>MSIITDVYAREILDSRGNPTIEVEVYTESGAFGRGMVPSGASTGEYEAVELRDGDKARYGGKGVTKAVDNVNNIIAEAIIGYDVRDQMAIDKAMIALDGTPNKGKLGANAILGVSIAVARAAADYLEVPLYHYLGGFNTKVLPTPMMNIINGGSHADNSIDFQEFMIMPVGAPTFKEALRMGAEVFHALAAILKSRGLATSVGDEGGFAPNLGSNEEGFEVIIEAIEKAGYVPGKDV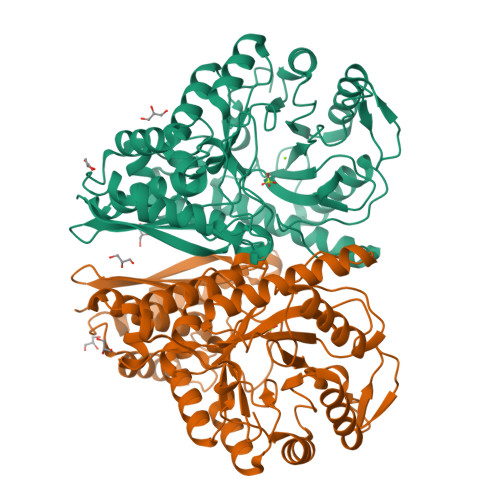VLAMDAASSEFYDKEKGVYVLADSGEGEKTTDEMIKFYEELVSKYPIISIEDGLDENDWDGFKKLTDVLGDKVQLVGDDLFVTNTQKLSEGIEKGIANSILIKVNQIGTLTETFEAIEMAKEAGYTAVVSHRSGETEDSTISDIAVATNAGQIKTGSLSRTDRIAKYNQLLRIEDQLGEVAEYKGLKSFYNLKAA[2x]>[2x]GPGAMERVLKVFHYFENSSEPTTWASIIRHGDATDVRGIIQKIVDCHKVKNVACYGLRLSHLQSEEVHWLHLDMGVSNVREKFELAHPPEEWKYELRIRYLPKGFLNQFTEDKPTLNFFYQQVKNDYMLEIADQVDQEIALKLGCLEIRRSYGEMRGNALEKKSNYEVLEKDVGLRRFFPKSLLDSVKAKTLRKLIQQTFRQFANLNREESILKFFEILSPVYRFDKECFKCALGSSWIISVELAIGPEEGISYLTDKGANPTHLADFNQVQTIQYSNSEDKDRKGMLQLKIAGAPEPLTVTAPSLTIAENMADLIDGYCRLVNGATQSFIIRPQKEGERALPSIPKLANNEKQGVRSHTVSVSETDDYAEIIDEEDTYTMPSTRDYEIQRERIELGRCIGEGQFGDVHQGIYMSPENPAMAVAIKTCKNCT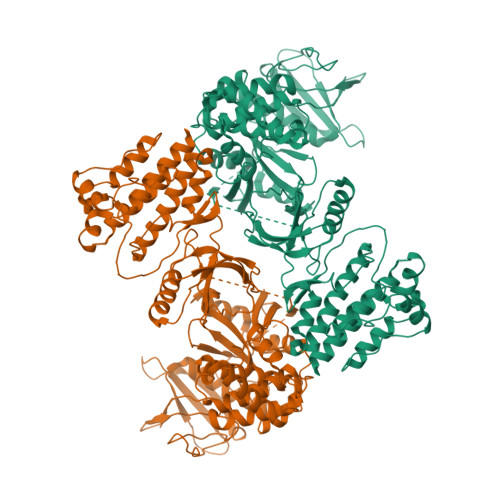SDSVREKFLQEALTMRQFDHPHIVKLIGVITENPVWIIMELCTLGELRSFLQVRKFSLDLASLILYAYQLSTALAYLESKRFVHRDIAARNVLVSATDCVKLGDFGLSRYMEDSTYYKASKGKLPIKWMAPESINFRRFTSASDVWMFGVCMWEILMHGVKPFQGVKNNDVIGRIENGERLPMPPNCPPTLYSLMTKCWAYDPSRRPRFTELKAQLSTILEEEKLQ>KSPIFGPEEVNSVEGNSVSITCYYPPTSVNRHTRKYWCRQGARGGCITLISSEGYVSSKYAGRANLTNFPENGTFVVNIAQLSQDDSG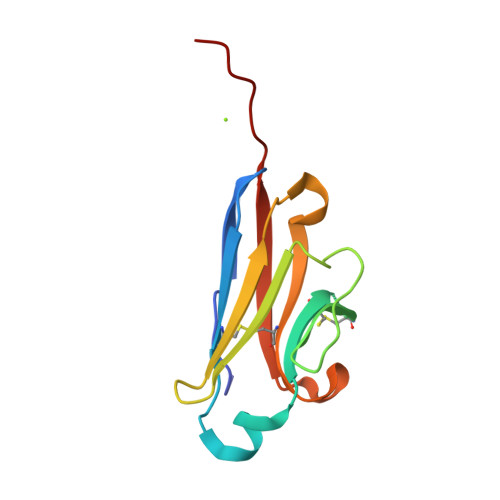RYKCGLGINSRGLSFDVSLEVLEHHHHHH[6x]>[6x]SELLQRCE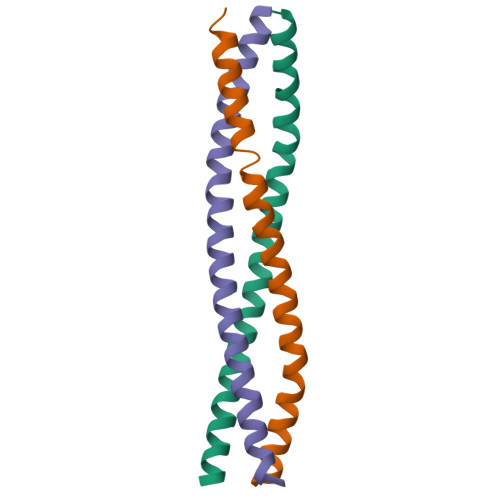SLEKKTATFENIVCVLNREVERVAMTAEACSRQHRLDQDKIEALSSKVQQLERSIGLEHHHHHH> GPGSGPVFVQEPSHVMFPLDSEEKKVKLSCEVKGNPKPHIRWKLNGTDVDIGMDFRYSVVDGSLLINNPNKTQDAGTYQCIATNSFGTIVSREAKLQFAYLENFKTRTRSTVSVRRGQGMVLLCGPPPHSGELSYAWIFNEYPSYQDNRRFVSQETGNLYIAKVEKSDVGNYTCVVTNTVTNHKVLGPPTPLILRNDGVMGEYEPKIEVQFPETVPAEKGTTVKLECFALGNPVPTILWRRADGKPIARKARRHKSNGILEIPNFQQEDAGSYECVAENSRGKNVAKGQLTFYAQPNWVQIINDIHVAMEESVFWECKANGRPKPTYRWLKNGDPLLTRDRIQIEQGTLNITIVNLSDAGMYQCVAENKHGVIFSSAELSVIAE;> GPGSGDPYWAYSGAYGPEHWVTSSVSCGGSHQSPIDILDHHARVGDEYQELQLDGFDNESSNKTWMKNTGKTVAILLKDDYFVSGAGLPGRFKAEKVEFHWGHSNGSAGSEHSVNGRRFPVEMQIFFYNPDDFDSFQTAISENRIIGA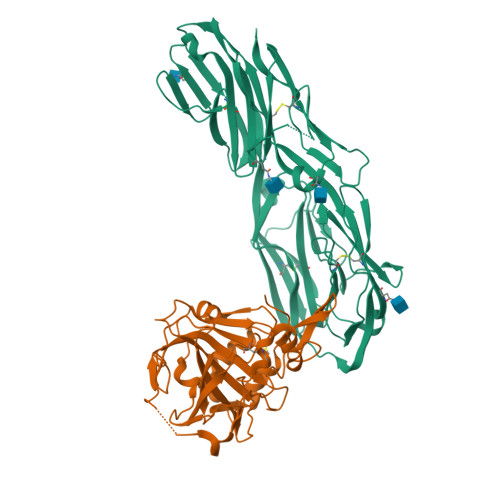MAIFFQVSPRDNSALDPIIHGLKGVVHHEKETFLDPFILRDLLPASLGSYYRYTGSLTTPPCSEIVEWIVFRRPVPISYHQLEAFYSIFTTEQQDHVKSVEYLRNNFRPQQALNDRVVSKS>[2x]MPAPHGGILQDLIARDALKKNELLSEAQSSDILVWNLTPRQLCDIELILNGGFSPLTGFLNENDYSSVVTDSRLADGTLWTIPITLDVDEAFANQIKPDTRIALFQDDEIPIAILTVQDVYKPNKTIEAERVFRGDPEHPAISYLFNVAGDYYVGGSLEAIQLPQHYDYPGLRKTPAQLRLEFQSRQWDRVVAFQTRNPMHRAHRELTVRAAREANAKVLIHPVVGLTKPGDIDHHTRVRVYQEIIKRYPNG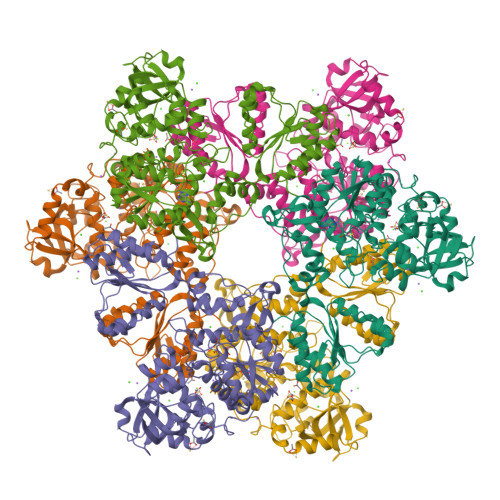IAFLSLLPLAMRMSGDREAVWHAIIRKNYGASHFIVGRDHAGPGKNSKGVDFYGPYDAQELVESYKHELDIEVVPFRMVTYLPDEDRYAPIDQIDTTKTRTLNISGTELRRRLRVGGEIPEWFSYPEVVKILRESNPPRPKQGFSIVLGNSLTVSREQLSIALLSTFLQFGGGRYYKIFEHNNKTELLSLIQDFIGSGSGLIIPDQWEDDKDSVVGKQNVYLLDTSSSADIQLESADEPISHIVQKVVLFLEDNGFFVF>[4x]MSKITINIKDNTIEYGHKEFVLSNLQEDIKNLAEI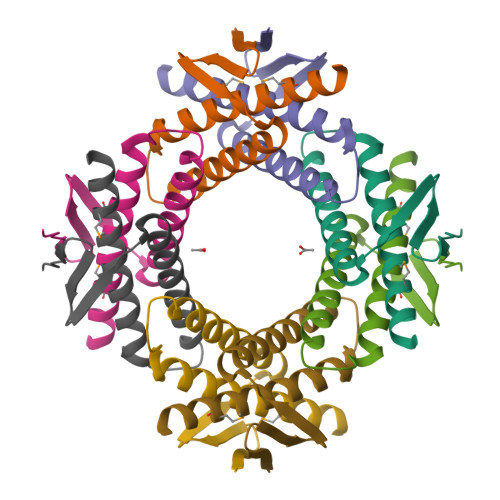VYQLAKLIEKLSQYEEEVDTELYNLLHEYAIYLAGATSMFIDSENKHHHHHH>[2x]ACCCGCAAGGCCGACGGC;>[2x]GCCGCCGCUG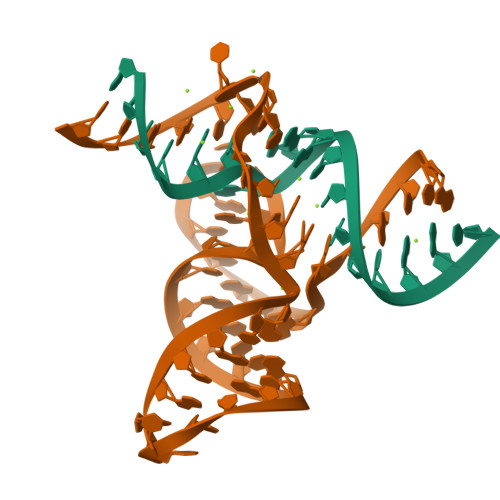GUGCAAGUCCAGCCACGCUUCGGCGUGGGCGCUCAUGGGU However, our results show that vc1313 encodes the MCP that senses d-Arg and d-Lys to initiate a repulsive chemotactic response in V. cholerae; therefore, we renamed this protein as MCPDRK for MCP sensing d-Arg (R) and d-Lys (K). MCPDRK contains a ligand binding domain (LBD) predicted to belong to the 4HB_MCP protein family (Pfam PF12729) as a sensory module, a transmembrane HAMP domain (Pfam PF00672) and a cytoplasmic MCP-signalling domain (Pfam PF00015) as output module. Overall, MCPDRK-LBD forms an antiparallel four-α-helix bundle structure (4HB). Here we reveal that d-arginine and d-lysine are chemotactic repellent signals for the cholera pathogen Vibrio cholerae. These d-amino acids are sensed by a single chemoreceptor MCPDRK co-transcribed with the racemase enzyme that synthesizes them under the control of the stress-response sigma factor RpoS.

To elucidate the molecular mechanisms of ligand recognition by MCPDRK, we purified the LBD domain of MCPDRK (20 kDa) with a Glutathione S-transferase (GST) tag that was cleaved off before the final size-exclusion chromatography (SEC) step. This purified LBD was monomeric in solution, both in the absence and presence of its d-Arg ligand, as determined by multi-angle laser light scattering (SEC-MALS). The crystals belonged to space group P1 and contained two LBD molecules, organized head-to-tail, in the asymmetric unit. As the monomers in the asymmetric unit were virtually identical and both were ligand bound, we here only show and discuss the A-chain of each structure. The final structure models correspond to residues 32–187 or 32–189 for the d-Arg and d-Lys-bound structures, respectively. In the MCPDRK-LBD structures, both d-Arg and d-Lys bind at the same site, at the bottom of the second and the third helix. To bind the ligands, Asp47 forms an ionic bond with the positively charged α-amine group of both DAAs. Further, Glu111 and Asp47 interact with the delocalized positive charge of the guanidino group from d-Arg; in a similar manner, the positively charged side-chain amine of d-Lys forms a salt bridge with Glu111. The ligands are further stabilized by hydrogen bonds with residues from all helices, namely Asn43, Thr48, Thr105, Glu111 and Asn176. Trp107, from the short loop between helix 2 and 3, forms a lid that closes off the binding site and has a stacking interaction with the ligands. Chemotaxis assays demonstrated the essentiality of 5 of the 7 MCPDRK-LBD residues tested (N43, T48, W107, E111 and N176) to promote a repulsive response to d-Arg in V. cholerae. d-Arg-mediated taxis was not affected by the N43A and T105A mutations, suggesting a less relevant role for these residues in stabilizing the d-Arg and d-Lys. MCPDRK’s d-Arg-binding pocket is located at the bottom of the second and the third helix, where only five residues are essential for recognizing this d-amino acid and similar compounds such as d-Lys.

>GPLGSSELDKIQSELLNYTDDTLPAMENVDAIKDKMSYWRRTQFAVLPMKDEAQIRQTIERNNRVQAEINDSLVAYGKTVWPGEEEQTFKRLMGNWNAYTAVTDQFNQTLLTQGADDAYPILANSLSTFEALESDFTLLIGILHQAMDSNKVQILSSVKTLNSTSEFPGRLERPHRD[2x]> MAEQVALSRTQVCGILREELFQGDAFHQSDTHIFIIMGASGDLAKKKIYPTIWWLFRDGLLPENTFIVGYARSRLTVADIRKQSEPFFKATPEEKLKLEDFFARNSYVAGQYDDAASYQRLNSHMNALHLGSQANRLFYLALPPTVYEAVTKNIHESCMSQIGWNRIIVEKPFGRDLQSSDRLSNHISSLFREDQIYRIDHYLGKEMVQNLMVLRFANRIFGPIWNRDNIACVILTFKEPFGTEGRGGYFDEFGIIRDVMQNHLLQMLCLVAMEKPASTNSDDVRDEKVKVLKCISEVQANNVVLGQYVGNPDGEGEATKGYLDDPTVPRGSTTATFAAVVLYVENERWDGVPFILRCGKALNERK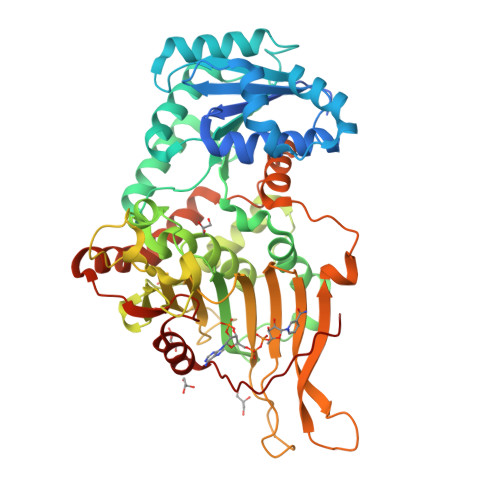AEVRLQFHDVAGDIFHQQCKRNELVIRVQPNEAVYTKMMTKKPGMFFNPEESELDLTYGNRYKNVKLPDAYERLILDVFCGSQMHFVRSDELREAWRIFTPLLHQIELEKPKPIPYIYGSRGPTEADELMKRVGFQYEGTYKWVNPHKL>MWRLRRAAVACEVCQSLVKHSSGIKGSLPLQKLHLVSRSIYHSHHPTLKLQRPQLRTSFQQFSSLTNLPLRKLKFSPIKYGYQPRRNFWPARLATRLLKLRYLILGSAVGGGYTAKKTFDQWKDMIPDLSEYKWIVPDIVWEIDEYIDFEKIRKALPSSEDLVKLAPDFDKIVESLSLLKDFFTSGSPEETAFRATDRGSESDKHFRKVSDKEKIDQLQEELLHTQLKYQRILERLEKENKELRKLVLQKDDKGIHHRKLKKSLIDMYSEVLDVLSDYDASYNTQDHLPRVVVVGDQSAGKTSVLEMIAQARIFPRGSGEMMTRSPVKVTLSEGPHHVALFKDSSREFDLTKEEDLAALRHEIELRMRKNVKEGCTVSPETISLNVKGPGLQRMVLVDLPGVINTVTSGMAPDTKETIFSISKAYMQNPNAIILCIQDGSVDAERSIVTDLVSQMDPHGRRTIFVLTKVDLAEKNVASPSRIQQIIEGKLFPMKALGYFAVVTGKGNSSESIEAIREYEEEFFQNSKLLKTSMLKAHQVTTRNLSLAVSDCFWKMVRESVEQQADSFKATRFNLETEWKNNYPRLRELDRNELFEKAKNEILDEVISLSQVTPKHWEEILQQSLWERVSTHVIENIYLPAAQTMNSGTFNTTVDIKLKQWTDKQLPNKAVEVAWETLQEEFSRFMTEPKGKEHDDIFDKLKE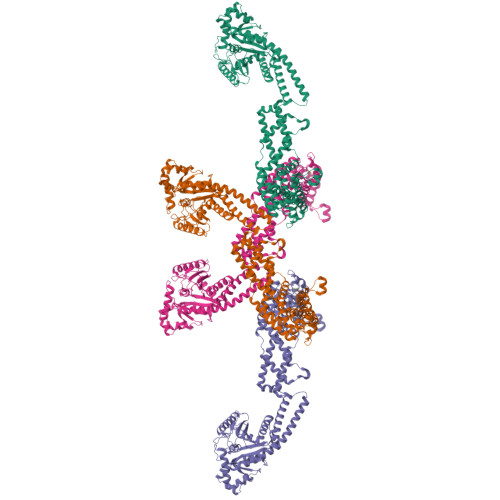AVKEESIKRHKWNDFAEDSLRVIQHNALEDRSISDKQQWDAAIYFMEEALQARLKDTENAIENMVGPDWKKRWLYWKNRTQEQCVHNETKNELEKMLKCNEEHPAYLASDEITTVRKNLESRGVEVDPSLIKDTWHQVYRRHFLKTALNHCNLCRRGFYYYQRHFVDSELECNDVVLFWRIQRMLAITANTLRQQLTNTEVRRLEKNVKEVLEDFAEDGEKKIKLLTGKRVQLAEDLKKVREIQEKLDAFIEALHQEK[4x]> TNMGLEAII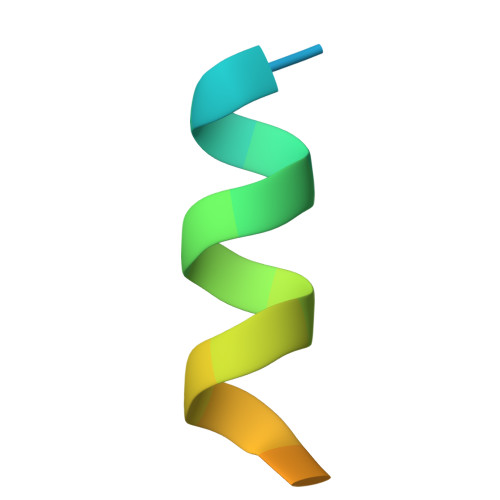RKALMGKYDQWEE>[2x]SAKDERAREILRGFKLNWMNLRDAETGKILWQGTEDLSVPGVEHEARVPKKILKCKAVSRELNFSSTEQMEKFRLEQKVYFKGQCLEEWFFEFGFVIPNSTNTWQSLIEAAPESQMMPASVLTGNVIIETKFFDDDLLVSTSRVRLFYV;>[2x]SSTIC

PDE6δ was shown to bind prenylated peptides or proteins of the Ras subfamily with approximately micromolar affinity and to play a critical role in their cellular distribution. INPP5E belongs to the inositol polyphosphate 5′-phosphatase family that hydrolyzes the 5′-phosphate of phosphatidylinositols and localizes to primary cilia. INPP5E contains a C-terminal CaaX motif where the C-terminal residue Cys644 is farnesylated. For certain membrane-associated, post-translationally modified proteins carrying an N-terminal myristoyl or a C-terminal prenyl motif, it has been shown that the import into cilia is dependent on the carrier proteins PDE6δ, UNC119a and UNC119b and on Arl3 as displacement factor.

The proteins show a hydrophobic cavity, where the farnesyl moieties of INPP5E and Rheb are inserted (upper). The prenyl groups overlay well and make an identical interaction pattern with the surrounding hydrophobic residues of PDE6δ (lower). However, the side chains of the residues on the −1 and −3 positions upstream of the farnesylated cysteine (the 0 position) in INPP5E and Rheb show different contacts with PDE6δ. As shown in Fig. 4b (upper), the serine side chain of Rheb on the −1 position makes a hydrogen bond with the side chain of glutamic acid (Glu88) from PDE6δ, whereas the hydrophobic side chain of the isoleucine of INPP5E at the equivalent position is situated in a highly hydrophobic environment mediated by five hydrophobic residues of PDE6δ (Val80, Trp90, Met118, Leu123 and Ile128). On the other hand, the lysine side chain of Rheb at the −3 position is pointing away from the binding pocket of PDE6δ, while the serine side chain of INPP5E at the equivalent position makes a hydrogen bond with the side chain of glutamic acid (Glu88) (lower). Thus, we reasoned that the different contact patterns of INPP5E and Rheb peptides with PDE6δ are responsible for the difference in affinities. Hence, we used a fluorescently labelled C-terminal farnesylated and carboxy-methylated peptide of INPP5E (residues 637–644) and Rheb (residues 175–181) to measure the affinity to PDE6δ by fluorescence polarization. Figure 1b (left) shows that PDE6δ binds to INPP5E peptide with low nanomolar affinity (Kd=3.7 nM±0.2,±indicates s.d., n=9). Analysis of the data with a competition model derived from the law of mass action as described1739 shows that the affinities to PDE6δ can be reversed, with a Kd values of (697±54 nM,±indicates s.d., n=14) for INPP5E(KS) and (12±2.7 nM,±indicates s.d., n=12) for Rheb(SI). Structural analysis revealed that the residues at the −1 and −3 positions relative to the farnesylated cysteine are the determinants for the binding affinity to PDE6δ.>GGAACCGGUGCGC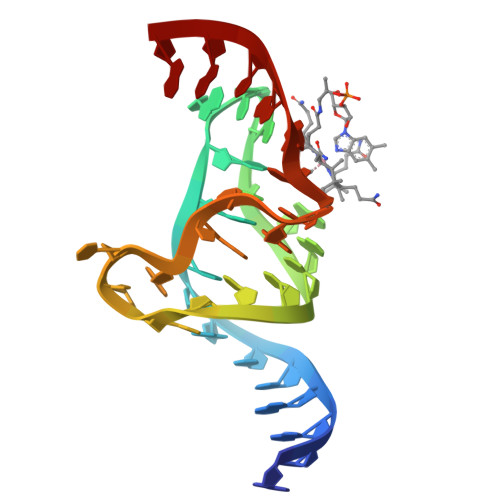AUAACCACCUCAGUGCGAGCAA[4x]>[12x]HCDLPCGVYDPAQARIEAESVKAVQEKMAGNDD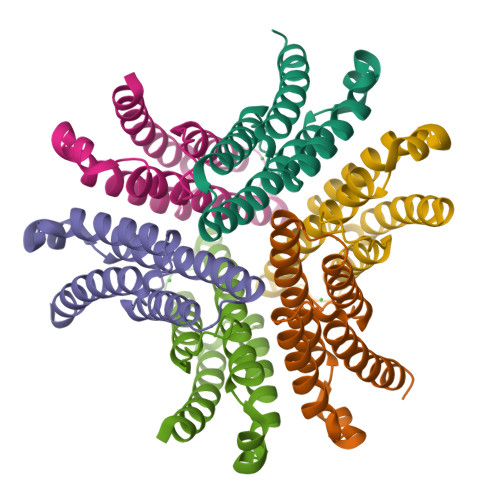PHFQTRATVIKEQRAELAKHHVSVLWSDYFKPPHFEKYPELHQLVNDTLKAMSAAKGSKDPATGQKALDYIAQIDKIFWETKKA Transcription factors (TFs) recognize specific bases within their DNA-binding motifs, with each base contributing nearly independently to total binding energy. However, the energetic contributions of particular dinucleotides can deviate strongly from the additive approximation, indicating that some TFs can specifically recognize DNA dinucleotides. Here we solved high-resolution (<1 Å) structures of MYF5 and BARHL2 bound to DNAs containing sets of dinucleotides that have different affinities to the proteins. The dinucleotides were recognized either enthalpically, by an extensive water network that connects the adjacent bases to the TF, or entropically, by a hydrophobic patch that maintained interfacial water mobility.

Mutation of the AC sequence led to a much larger loss of affinity than mutation of TT. Mutating the A7 to either G or C of DNAAC resulted in a loss of most water-mediated contacts and a very low affinity. Both DNAGC and DNACC complexes showed only one water molecule in the interface connecting the side-chain oxygens of Thr285 and Asn282 with the N4 of C18 or O6 of G18, respectively. Furthermore, neither complex retained the hydrophobic contacts involving either Thr278 or Thr285, further explaining their very low affinity.

>[5x]PRKARTAFSDHQLNQLERSFERQKYLSVQDRMDLAAALNLTDTQVKTWYQNRRTKWKRQTAV> GSHMGSADEERDHWQQFYFLSKRRRNLLRNPCGEEDLEGWSDVEHGGDGWKVEELPGDNGVEFTQDDSVKKYFASSFEWC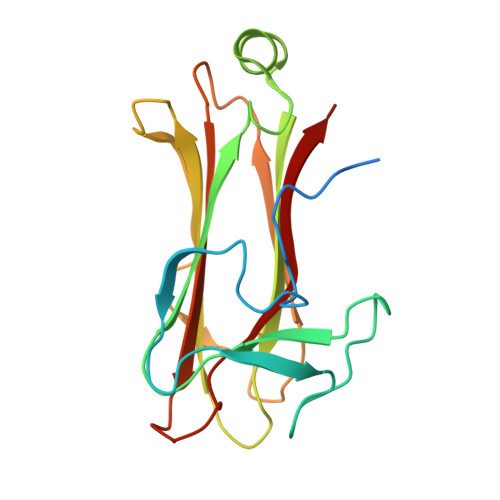RKAQVIDLQAEGYWEELLDTTQPAIVVKDWYSGRTDAGSLYELTVRLLSENEDVLAEFATGQVAVPEDGSWMEISHTFIDYGPGVRFVRFEHGGQDSVYWKGWFGARVTNSSVWVEP>MPAIFTHEGKVEGVPGNYP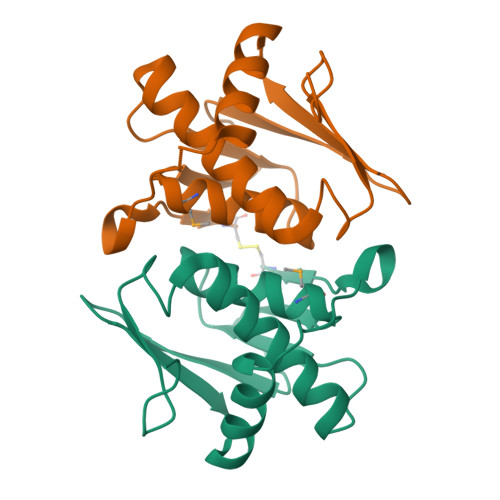LTAENLFRIGLALCTLWILDKEIEEPTLSIPETNFVTLALSVGFMNAGGSVNVGKGGDIKLFLQKGEIYVLEFQPLSETDIKKLESILFGRAPIPKKTGEDIGSFKC[2x]>[10x]MAAQNEQRPERIKTTPYLEGDVLSSDSGPLLSVFALQEIMQKVRQVQADYMTATREVDFTVPDVQKILDDIKALAAEQVYKIVKVPSISFRHIVMQSRDRVLRVDTYYEEMSQVGDVITEDEPEKFYSTIIKKVRFIRGKGSFILHDIPTRDHRGMEVAEPEVLGVEFKNVLPVLTAEHRAMIQNALDGSIIENGNVATRDVDVFIGACSEPVYRIYNRLQGYIEAVQLQELRNSIGWLERLGHRKRITYSQEVLTDFRRQDTIWVLALQLPVNPQVVWDVPRSSIANLIMNIATCLPTGEYIAPNPRISSITLTQRITTTGPFAILTGSTPTAQQLNDVRKIYLALMFPGQIILDLKIDPGERMDPAVRMVAGVVG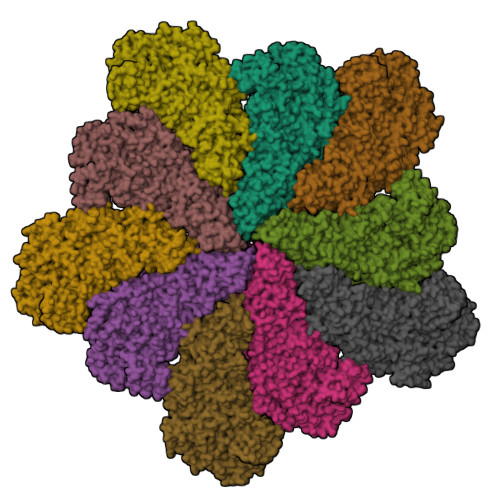HLLFTAGGRFTNLTQNMARQLDIALNDYLLYMYNTRVQVNYGPTGEPLDFQIGRNQYDCNVFRADFATGTGYNGWATIDVEYREPAPYVHAQRYIRYCGIDSRELINPTTYGIGMTYHCYNEMLRMLVAAGKDSEAAYFRSMLPFHMVRFARINQIINEDLHSVFSLPDDMFNALLPDLIAGAHQNADPVVLDVSWISLWFAFNRSFEPTHRNEMLEVAPLIESVYASELSVMKVDMRHLSLMQRRFPDVLIQARPSHFWKAVLNDSPEAVKAVMNLSHSHNFINIRDMMRWVMLPSLQPSLKLALEEEAWAAANDFEDLMLTDQVYMHRDMLPEPRLDDIERFRQEGFYYTNMLEAPPEIDRVVQYTYEIARLQANMGQFRAALRRIMDDDDWVRFGGVLRTVRVKFYDARPPDDVLQGLPFSYDTNERGGLAYATIKYATETTIFYLIYNVEFSNTPDSLVLINPTYTMTKVFINKRIVERVRVGQILAVLNRRFVAYKGKMRIMDITQSLKMGTKLAAPTV> RVQSGKINCGDDAGWAKVPSDDPGRDNTRELAKNITFA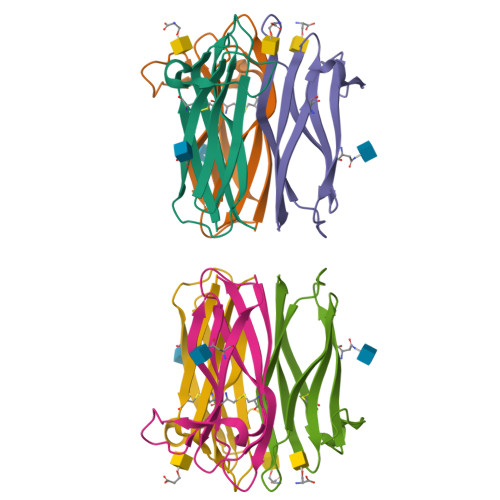SPYCRPPVVLLSITQLDVEQSQNLRVIARLYSVSPTGFKASCYTWHNTKVYSMSISWISIENY>DDATADSRKTYTLTDYLKNTYRLKLYSLRWISDHEYLYKQENNILVFNAEYGNSSVFLENSTFDEFGHSINDYSISPDGQFILLEYNYVKQWRHSYTASYDIYDLNKRQLITEERIPNNTQWVTWSPVGHKLAYVWNNDIYVKIEPNLPSYRITWTGKEDIIYNGITDWVYEEEVFSAYSALWWSPNGTFLAYAQFNDT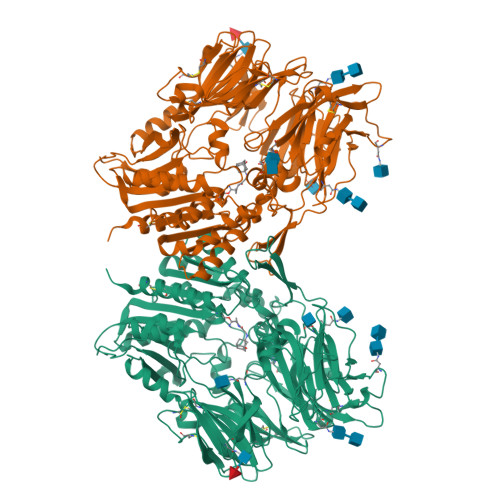EVPLIEYSFYSDESLQYPKTVRVPYPKAGAVNPTVKFFVVNTDSLSSVTNATSIQITAPASMLIGDHYLCDVTWATQERISLQWLRRIQNYSVMDICDYDESSGRWNCLVARQHIEMSTTGWVGRFRPSEPHFTLDGNSFYKIISNEEGYRHICYFQIDKKDCTFITKGTWEVIGIEALTSDYLYYISNEYKGMPGGRNLYKIQLSDYTKVTCLSCELNPERCQYYSVSFSKEAKYYQLRCSGPGLPLYTLHSSVNDKGLRVLEDNSALDKMLQNVQMPSKKLDFIILNETKFWYQMILPPHFDKSKKYPLLLDVYAGPCSQKADTVFRLNWATYLASTENIIVASFDGRGSGYQGDKIMHAINRRLGTFEVEDQIEAARQFSKMGFVDNKRIAIWGWSYGGYVTSMVLGSGSGVFKCGIAVAPVSRWEYYDSVYTERYMGLPTPEDNLDHYRNSTVMSRAENFKQVEYLLIHGTADDNVHFQQSAQISKALVDVGVDFQAMWYTDEDHGIASSTAHQHIYTHMSHFIKQCFSLPHHHHHH[2x]>GPHMADDVVITARNNGPYHIKGSFRIVTQGGRELPVEQGQAWLCRCGHSLNKPFCDGSHKRVEFDSNLD[2x]

The recently discovered CDGSH iron-sulfur domains (CISDs) are characterized by one or two highly conserved 17-residue CDGSH motifs with a consensus sequence of [ΦCXCXX(S/T)XXXPΦCDG(S/T/A)H], where Φ and X are a hydrophobic or any residue, respectively. The [2Fe-2S] cluster is coordinated with three cysteine residues and one histidine residue in the CDGSH motif. We synthesized genes for a type 3 CISD (PcCISD) from Pyrobaculum calidifontis, which is a hyperthermophilic archaeon, a type 4 CISD (RsCISD) from Ralstonia solanacearum, which is a soil-born plant pathogenic bacterium, and a type 6 CISD (MmCISD) from Magnetospirillum magneticum, which is an aquatic alphabacterium that utilizes iron reduction to derive energy. The four CISD structures display striking similarity in their overall appearance, with dual iron-sulfur binding modules and a β-sandwich dimerization module.

RsCISD adopts an intertwined dimeric structure with the dimer interface burying 1250 Å2 of solvent accessible area per monomer. Residues 6–66 of RsCISD are resolved in the structure and form five consecutive β-strands (β1 though β5) followed by the iron-sulfur binding module and a short α-helix, α1. Each subunit binds a [2Fe-2S] cluster via residues Cys41, Cys43, Cys52 and His56 in the CDGSH motif. The structure contains a β-sandwich packed by two intermolecular five-stranded β-sheets. Each β-sheet comprises strands β1, β2 and β5 from one subunit and strand β3′ and β4′ from the other subunit with the order β5-β2-β1-β3′-β4′ (prime denotes the other subunit). The intermolecular pairing between strand β1 and β3′ is parallel, whereas all other adjacent strand pairing is antiparallel. The β-sandwich is stabilized by a large number of hydrophobic residues (Ile7, Ala9, Tyr15, Ile17, Phe21, Ile23, Leu31, Ala38, Leu40, Pro50 and Phe51), which are highly conserved in type 4 CISDs. The two iron-sulfur binding modules are packed closer to each other in the RsCISD structure than in the mitoNEET and MmCISD structures. The interface between the two iron-sulfur binding modules is mainly polar, burying two arginine residues and four water molecules. Lys57 is located at the opening of the [2Fe-2S] cluster and is conserved as lysine or arginine in more than 90% type 4 CISDs and thus may be functionally important.>SKKPRQKRTATKAYNVTQAFGRRGPEQTQGNFGDQELIRQGTDYKHWPQIAQFAPSASAFFGMSRIGMEVTPSGTW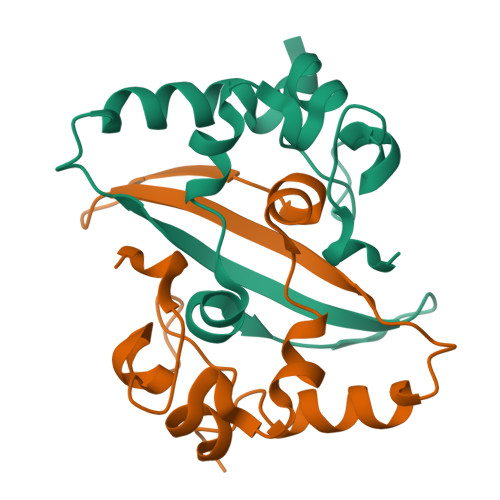LTYTGAIKLDDKDPNFKDQVILLNKHIDAYKT[12x]> QDADKLPHTKVTLVAPPQVHPHEQATKSGPKVVEFTMTIEEKKMVIDDKGTTLQAMTFNGSMPGPTLVVHEGDYVQLTLVNPATNAMPHNVDFHGATGALGGAKLTNVNPGEQATLRFKADRSGTFVYVCAPEGMVPWHVVSGMSGTLMVLPRDGLKDPQGKPLHYDRAYTIGEFDLYIPKGPDGKYKDYATLAESYGDTVQVMRTLTPSHIVFNGKVGALTGANALTAKVGETVLLIHSQANRDTRPHLIGGHGDWVWETGKFANPPQRDLETWFIRGGSAGAALYTFKQPGVYAYLNHNLIEAFELGAAGHIKVEG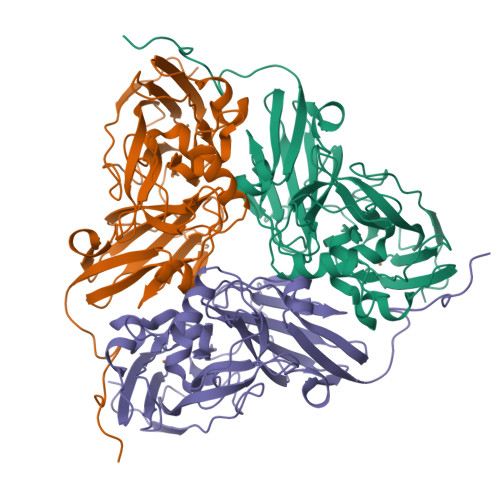KWNDDLMKQIKAPAPIPR>[6x]ASMLPQVKALYPYTAANDEELSFKVGDIITILEKDEGWWKGELNGQEGWIPNNYV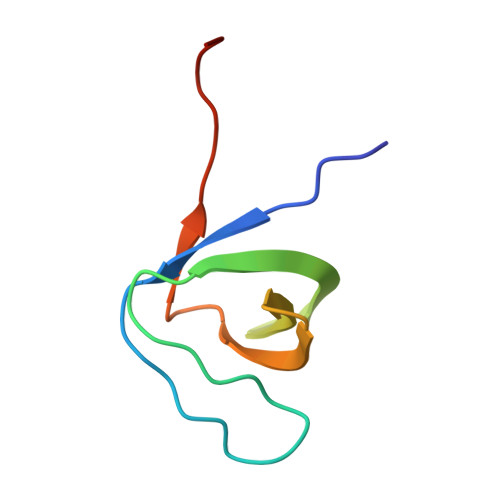KEILEHHHHHH> MGSSHHHHHHSQDPMPRVVPDQRSKFENEEFFRKLSRECEIKYTGFRDRPHEERQARFQNACRDGRSEIAFVATGTNLSLQFFPASWQGEQRQTPSREYVDLEREAGKVYLKAPMILNGVCVIWKGWIDLQRLDGMGC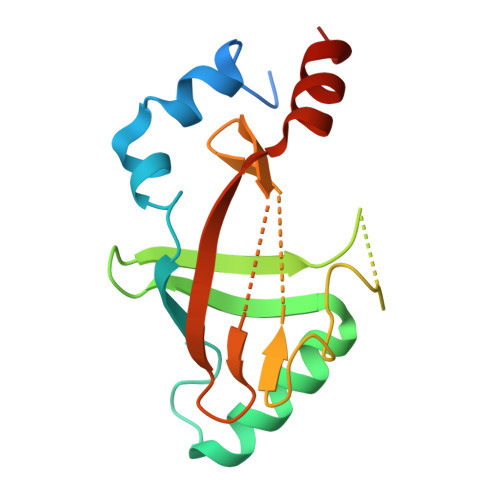LEFDEERAQQEDALAQQA>ATGSRPRDCLDVLLSGQQDDGVYSVFPTHYPAGFQVYCDMRTDGGGWTVFQRREDGSVNFFRGWDAYRDGFGRLTGEHWLGLKRIHALTTQAAYELHVDLEDFENGTAYARYGSFGVGLFSVDPEEDGYPLTVADYSGTAGDSLLKHSGMRFTTKDRDSDHSENNCAAFYRGAWWYRNCHTSNLNGQYLRGA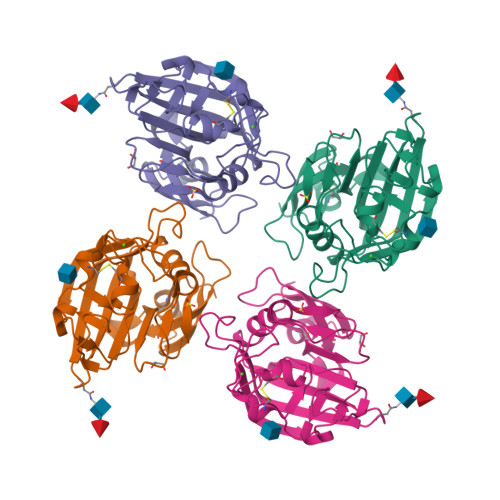HASYADGVEWSSWTGWQYSLKFSEMKIRPVREDR[2x]> EPPLVFEPVTLE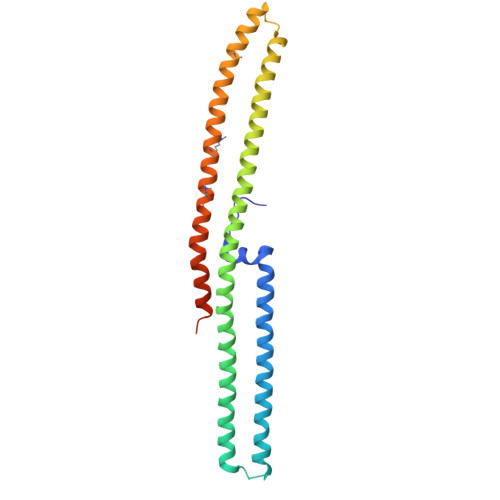SLRQEKGFQKVGKKQIKELDTLRKKHAKERTSVQKTQNAAIDKLIKGKSKDDIRNDANIKNSINDQTKQWTDMIARHRKEEWDMLRQHVQDSQDAMKALMLTVQAAQIKQLEDRHARDIKDLNAKQAKMSADTAKEVQNDKTLKTKNEKDRRLREKRQNNVKRFMEEKKQIGVKQGRAMEKLKLAHSKQIEEFSTDVQKLMDMYKIEEEAYKTQGKTEFYA> KAHVLAASVEQATENFLEKGDKIAKESQFLKEELVVAVEDVRKQGDLMKSAAGEFADDPCSSVKRGNMVRAARALLSAVTRLLILADMADVYKLLVQLKVVEDGILKLRNAGN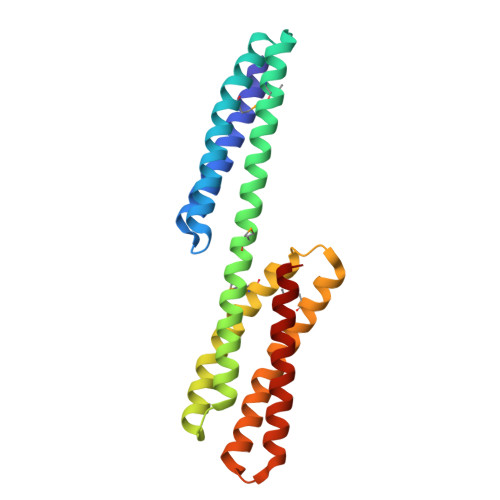EQDLGIQYKALKPEVDKLNIMAAKRQQELKDVGNRDQMAAARGILQKNVPILYTASQACLQHPDVAAYKANRDLIYKQLQQAVTGISNAAQA>[2x]SKINV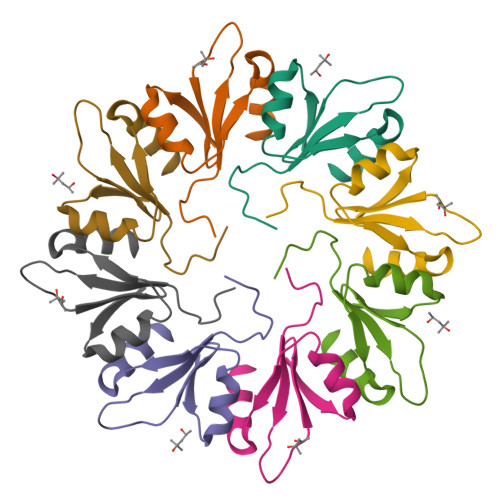NVENVSGVQGFLFHTDGKESYGYRAFINGVEIGIKDIETVQGFQQIIPSINISKSDVEAIKKAMKK> GKPLVVTTIGMIADAVKNIAQGDVHLKGLMGPGVDPHLYTATAGDVEWLGNADLILYNGLHLETKMGEVFSKLRGSRLVVAVSETIPV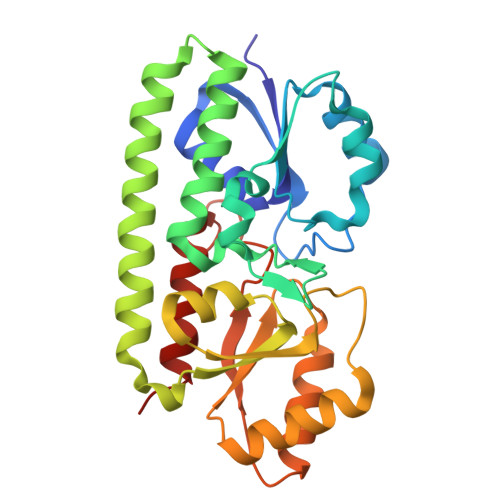SQRLSLEEAEFDPHVWFDVKLWSYSVKAVYESLCKLLPGKTREFTQRYQAYQQQLDKLDAYVRRKAQSLPAERRVLVTAHDAFGYFSRAYGFEVKGLQGVSTASEASAHDMQELAAFIAQRKLPAIFIESSIPHKNVEALRDAVQARGHVVQIGGELFSDAMGDAGTSEGTYVGMVTHNIDTIVAALAR CFH and CFHR proteins are encoded by adjacent genes and form a protein family. CFHR proteins are composed of four to nine complement control protein domains, also called short consensus repeats, and the two most C-terminal domains have relatively high sequence homologies to the C-terminal domains of CFH. There are only two residues that are different in the last two C-terminal domains of CFH and CFHR1 (domains 19–20 and 4–5, respectively). Domains 19 and 20 of CFH are responsible for directing its complement regulatory activity to cell and extracellular matrix surfaces by binding simultaneously to both C3b and negatively charged glycosaminoglycans or sialic acid glycans on the surfaces.

Patients with the autoimmune form of aHUS nearly always lack certain CFH-related proteins, primarily CFHR1 (CFH-related protein-1). CFH-AAs often cross-react with CFHR1 (13, 15, 26), but the exact location of the autoantibody site on CFHR1 has not been determined. We found structural differences in the autoantibody-binding site of CFH domain 20 and the corresponding homologous site of CFHR1 domain 5. Also, the hydrogen bonds stabilizing the loop in CFH and CFHR1 are clearly different. Second, there are no direct contacts between the residues of the CFH-AA site (Arg-281–Leu-288) and the molecule in the neighboring crystal cell. Our results suggest that the reason for the functional difference between the most C-terminal domains of CFH and CFHR1 is their varied ability to bind to heparin or glycosaminoglycans on self-cells because the loop that has a different conformation in CFH and CFHR1 contains several of the heparin-binding residues. In this model, called the “induced neoepitope model,” the normal structure of the Arg-1182–Leu-1189 loop of CFH can be turned into an autoantigenic conformation upon induction by at least one microbial ligand binding to that region of CFH domain 20. Our model provides an explanation as to why immunization against the CFH-AA site could occur only in CFHR1-deficient individuals because, in normal individuals, the presence of CFHR1 with an epitope similar to the hypothetical induced autoantigenic conformation of CFH would have guaranteed tolerance to that conformation of CFH. Cumulatively, our data suggest that association of CFHR1 deficiency with autoimmune aHUS could be due to the structural difference between CFHR1 and the autoantigenic CFH epitope, suggesting a novel explanation for CFHR1 deficiency in the pathogenesis of autoimmune aHUS.

>[2x]TGKCGPPPPIDNGDITSFPLSVYAPASSVEYQCQNLYQLEGNKRITCRNGQWSEPPKCLHPCVISREIMENYNIALRWTAKQKLYLRTGESAEFVCKRGYRLSSRSHTLRTTCWDGKLEYPTCAK> KKAVINGEQIRSISDLHQTLKKELALPEYY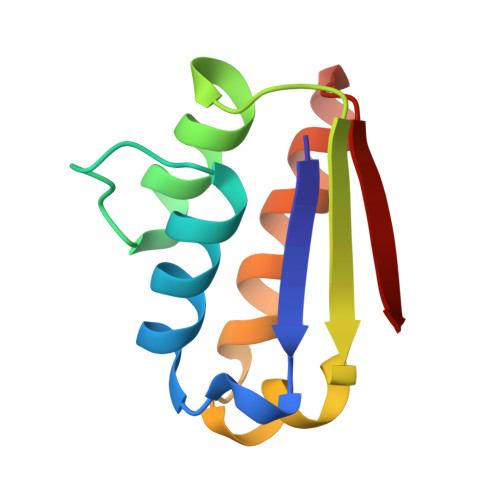GENLDALWDALTGWVEYPLVLEWRQFEQSKQLTENGAESVLQVFRAAKAEGADITIILS2-chloro-N-[4-({5-fluoro-2-[(4-hydroxyphenyl)amino]pyrimidin-4-yl}amino)phenyl]benzamide 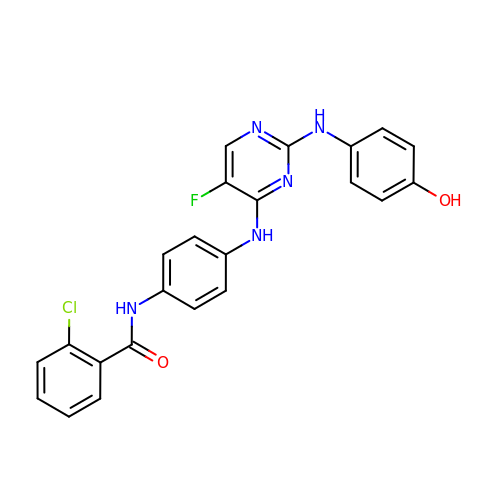| C23 H17 Cl F N5 O2 | ZYURNHOEBWWJHI-UHFFFAOYSA-N> MAHHHHHHNPNYCFAGKTSSISDLKEVPRKNITLIRGLGHGAFGEVYEGQVSGMPNDPSPLQVAVKTLPEVCSEQDELDFLMEALIISKFNHQNIVRCIGVSLQSLPRF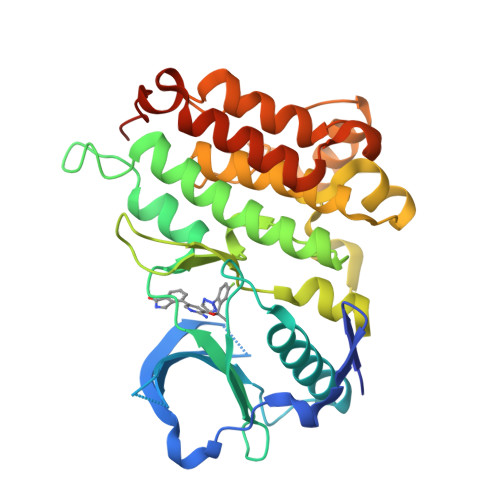ILLELMAGGDLKSFLRETRPRPSQPSSLAMLDLLHVARDIACGCQYLEENHFIHRDIAARNCLLTCPGPGRVAKIGDFGMARDIYRASYYRKGGCAMLPVKWMPPEAFMEGIFTSKTDTWSFGVLLWEIFSLGYMPYPSKSNQEVLEFVTSGGRMDPPKNCPGPVYRIMTQCWQHQPEDRPNFAIILERIEYCTQDPDVINTALPIEYGPLVEEEEKV3-[4-(2-METHYL-IMIDAZO[4,5-C]PYRIDIN-1-YL)BENZYL]-3H-BENZOTHIAZOL-2-ONE | C21 H16 N4 O S | 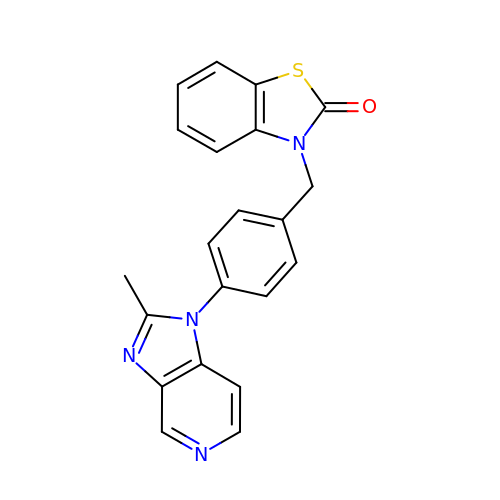WUOLYUKMMRCXGH-UHFFFAOYSA-N> PNIEMFVVEGLSDQQKEKLIDALTAATV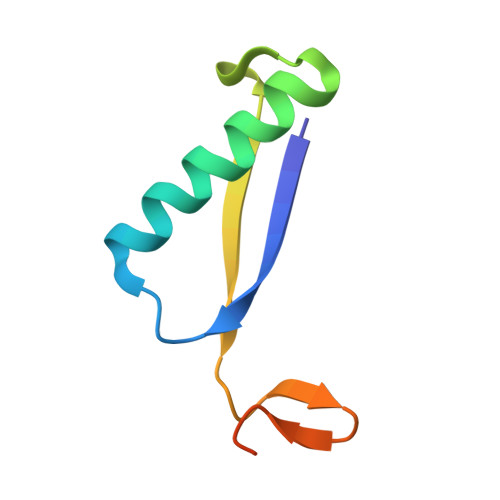EAIDAPADSIRVWLSEIPAKQFGIAGKSVAAIEAARKNK> GSHMPTTAASTPDAVDKYLETPGDENEHAHFQKAKERLEAKHRERMSQVMREWEEAERQAKNLPKADKKAVIQHFQEKVESLEQEAANERQQLVETHMARVEAMLNDRRRLALENYITALQAVPPRPRHVFNMLKKYVRAEQKDRQHTLKHFEHVRMVD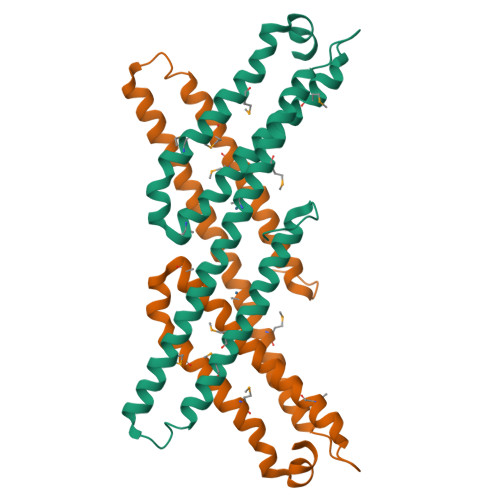PKKAAQIRSQVMTHLRVIYERMNQSLSLLYNVPAVAEEIQDEVDELLQ> MSQSPRRIILS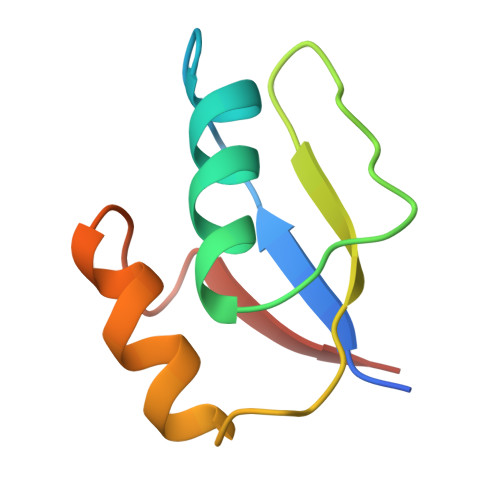RLKAGEVDLLEEELGHLTTLTDVVKGADSLSAILPGDIAEDDITAVLCFVIEADQITFETVEV> ATIKDVAKR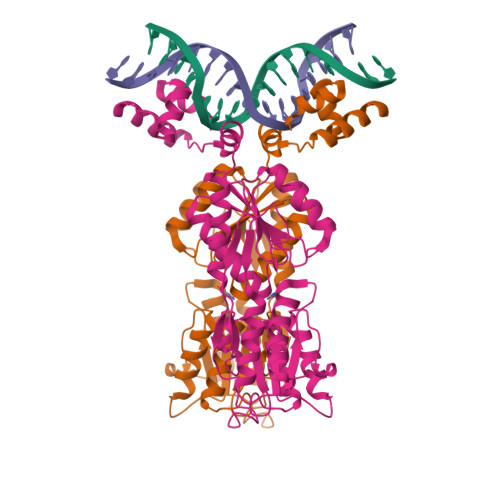ANVSTTTVSHVINKTRFVAEETRNAVWAAIKELHYSPSAVARSLKVNHTKSIGLLATSSEAAYFAEIIEAVEKNCFQKGYTLILGNAWNNLEKQRAYLSMMAQKRVDGLLVMCSEYPEPLLAMLEEYRHIPMVVMDFGEAKADFTDAVIDNAFEGGYMAGRYLIERGHREIGVIPGPLERNTGAGRLAGFMKAMEEAMIKVPESWIVQGDFEPESGYRAMQQILSQPHRPTAVFCGGDIMAMGALCAADEMGLRVPQDVSLIGYDNVRNARYFTPALTTIHQPKDSLGETAFNMLLDRIVNKREEPQSIEVHPRLIERRSVADGPFRDYRR4-amino-7-methyl-2-({5-methyl-1-[(3R)-oxolan-3-yl]-1H-pyrazol-4-yl}amino)-6-[(2R)-2-methylpyrrolidin-1-yl]-7H-pyrrolo[2,3-d]pyrimidine-5-carbonitrile 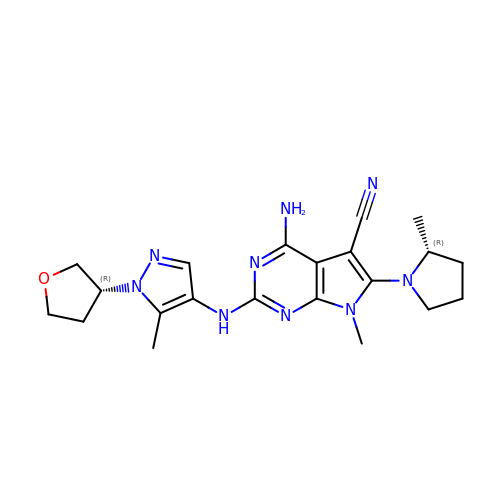| C21 H27 N9 O | QSDVZPULRUJSBC-TZMCWYRMSA-N> LMFNEVDDMKSHKLNAFSYMNKSDSTTLKNMAKDLKIYVTPINMYKENERLYDLKQKTSLITDDEDRLNKIEDIEDRQKKLESINEVFEKQAGIFFDKNYPDQSLNYSDDEKIFITRTILNDRDVLPANNELEDIVKEKRIKEAQISLNTVLGNRDISLESIAAASNFFADKLSNILEKNNLSFDDVLENKHEGMEDSLKIDYYTNKLEVFRNAENILEDYYDVQIKELFTDDEDYKAFNEVTDIKEKQQLIDFKTYHGTENTIEMLETGNFIPKYSDEDRKYITEQVKLLQEKEFKPNKNQHDKFVFGAIQKKLLSE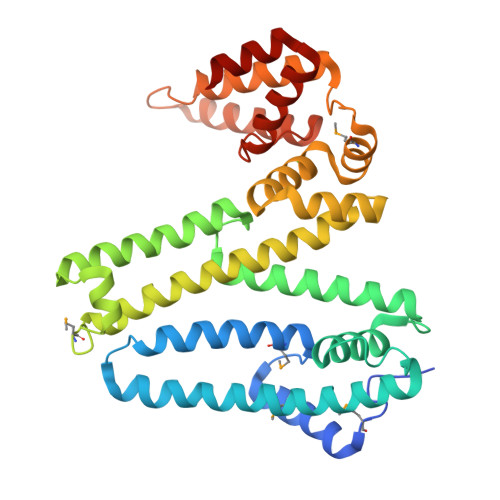YDFDYSDNNDLKHLYQESNEVGDEISKDNIEEFYE>MPGFELFGPEEKQEVADVMEHGFTFRYNFDHMRNDRWKTRDMEQLLCEKMNVKHAHLLSSGTAALQTAMMAAGIGAGDEVIVPPFTFVASVEAIFMAGAVPIFAEIDETLCLSPEGIEAVITPRTKAINLVHMCGSMAKMDEIKAICKKHNLVLLEDACQAIGGSYKGQALGTIGDVGCYSFDSVKTITCGEGGAVITNNTEIYDNAHMFSDHGHDHIGKDRGAESHPIMGLNFRISEMNAALGLAQLRKLDTIIDIQRKNKKAIKDAMASIPEVSFREIPDPEGDSAGFLSFMLPTEARTQEISKKLAANGVDGCFYWYVNNWHYLKN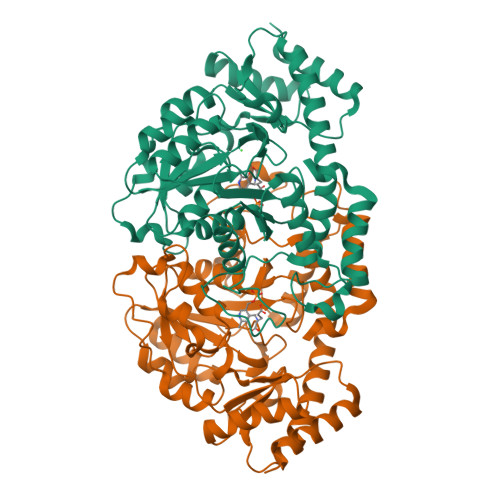WKHIQELKAPAALPITLIADRPDYTQISVPKSDAIMSRTISMLIKLSWTDAQIAERIENIKKAFAQLEHHHHHH[4x]>AAGAPKPPQEPDMNNLPENPIPQHQAKFVLNTIKAVKRNREAVPFLHPVDTVKLNVPFYYNYIPRPMDLSTIERKINLKAYEDVSQVVDDFNLMVKNCKKFNGEAAGISKMATNIQAQFEKLMVKVPPKELPAGTNV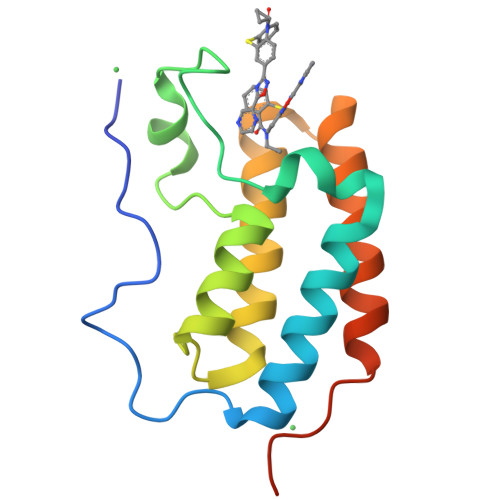A[4x]>[3x]MKNEKLAKGEMNLNALFIGDKAENGQLYKDLLIDLVDEHLGWRQNYMPQDMPVISSQERTSKSYEKTVNHMKDVLNEISSRMRTHSVPWHTAGRYWGHMNSETLMPSLLAYNFAMLWNGNNVAYESSPATSQMEEEVGHEFAHLMSYKNGWGHIVADGSLANLEGLWYARNIKSLPFAMKEVKPELVAGKSDWELLNMPTKEIMDLLESAEDEIDEIKAHSARSGKHLQAIGKWLVPQTKHYSWLKAADIIGIGLDQVIPVPVDHNYRMDINELEKIVRGLAEEQIPVLGVVGVVGSTEEGAVDSIDKIIALRDELMKDGIYYYVHVDAAYGGYGRAIFLDEDNNFIPYEDLQDVHEEYGVFKEKKEHISREVYDAYKAIELAESVTIDPHAMGYIPYSAGGIVIQDIRMRDVISYFATYVFEKGADIPALLGAYILEGSKAGATAASVWAAHHVLPLNVAGYGKLIGASIEGSHHFYNFLND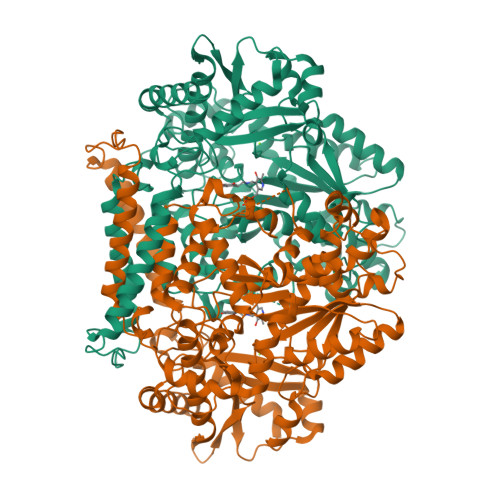LTFKVGDKEIEVHTLTHPDFNMVDYVFKEKGNDDLVAMNKLNHDVYDYASYVKGNIYNNEFITSHTDFAIPDYGNSPLKFVNSLGFSDEEWNRAGKVTVLRAAVMTPYMNDKEEFDVYAPKIQAALQEKLEQIYDVK>MAYG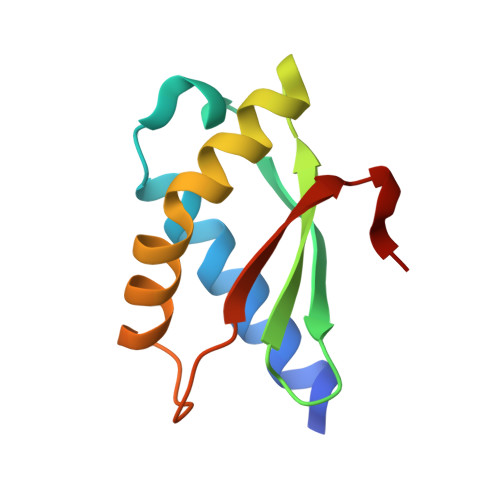KAHLEAQLKRALAEEIQALEDPRLFLLTVEAVRLSKDGSVLSVYVEAFREEEGALRALSRAERRLVAALARRVRMRRLPRLEFLPWRASPA[2x]>LTEQQRRELDWEKTDGLMPVIVQHAVSGEVLMLGYMNPEALDKTIESGKVTFFSRTKQRLWIKGETSGNFLNVVSIAPDCDNDTLLVLANPIGPTCHKGTSSCFGNTAHQWLFLYQLEQLLAERKYADPETSYTAKLYASGTKRIAQKVGEEGVETALAATVHDRFELTNEASDLMYHLLVLLQDQDLDLT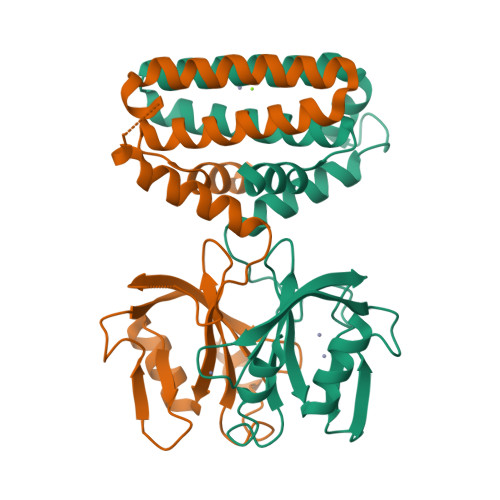TVIENLHKRHQ[2x]>[4x]GMTTFTLDERLERDGIPIGTLGLCQMRLMNDRRWPWLILVPQRADIKEVFELTPLDQAMLT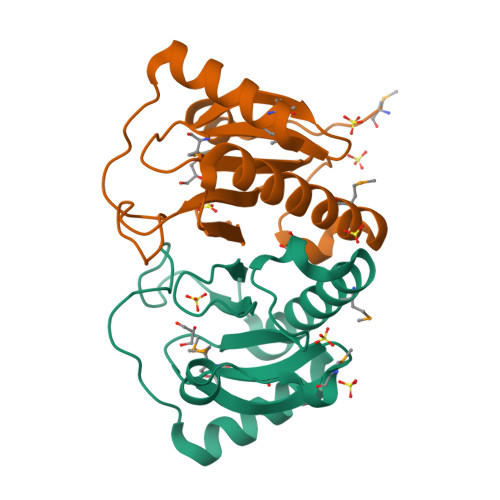FETNLVAAGLKKATGAEKINIGALGNIVRQLHVHVIARREGDPNWPGPVWGFGKAEPWPEEEHRTFAARIMENL> SSLQGPELHGWRPPVDCVRANELCAAESNCSSRYRTLRQCLAGRDRNTMLANKECQAALEVLQESPLYDCRCKRGMKKELQCLQIYWSIHLGLTEGEEFY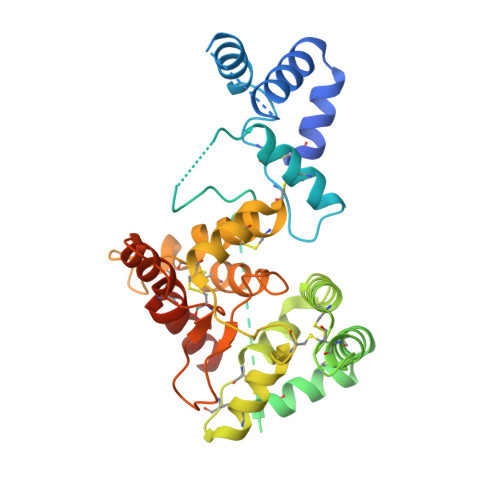EASPYEPVTSRLSDIFRLASIFSGTGADPVVSAKSNHCLDAAKACNLNDNCKKLRSSYISICNREISPTERCNRRKCHKALRQFFDRVPSEYTYRMLFCSCQDQACAERRRQTILPSCSYEDKEKPNCLDLRGVCRTDHLCRSRLADFHANCRASYQTVTSCPADNYQACLGSYAGMIGFDMTPNYVDSSPTGIVVSPWCSCRGSGNMEEECEKFLRDFTENPCLRNAIQAFGNGTDVNGTHHHHHHHH> SNAGGSATGTGLVYVDAFTRFHCLWDASHPECPARVSTVMEMLETEGLLGRCVQVEARAVTEDELLLVHTKEYVELMKSTQNMTEEEL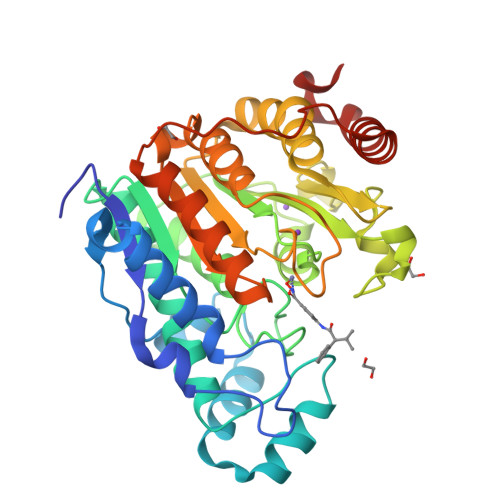KTLAEKYDSVYLHPGFFSSACLSVGSVLQLVDKVMTSQLRNGFSINRPPGHHAQADKMNGFCMFNNLAIAARYAQKRHRVQRVLIVDWDVHHGQGIQYIFEEDPSVLYFSVHRYEDGSFWPHLKESDSSSVGSGAGQGYNINLPWNKVGMESGDYITAFQQLLLPVAYEFQPQLVLVAAGFDAVIGDPKGGMQVSPECFSILTHMLKGVAQGRLVLALEGGYNLQSTAEGVCASMRSLLGDPCPHLPSSGAPCESALKSISKTISDLYPFWKSLQTFE(1~{R},2~{S},4~{S},5~{R})-cyclohexane-1,2,3,4,5-pentol 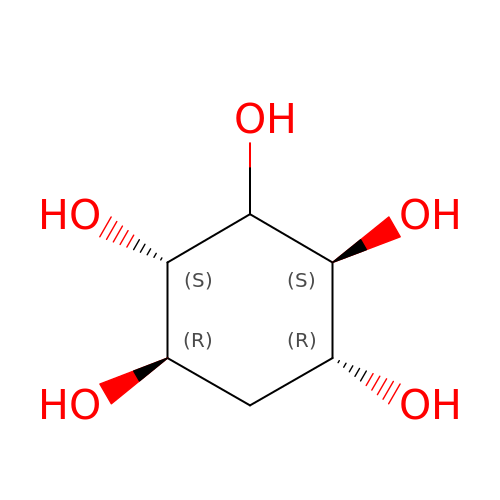| C6 H12 O5 | IMPKVMRTXBRHRB-MBMOQRBOSA-N> CCAGGCC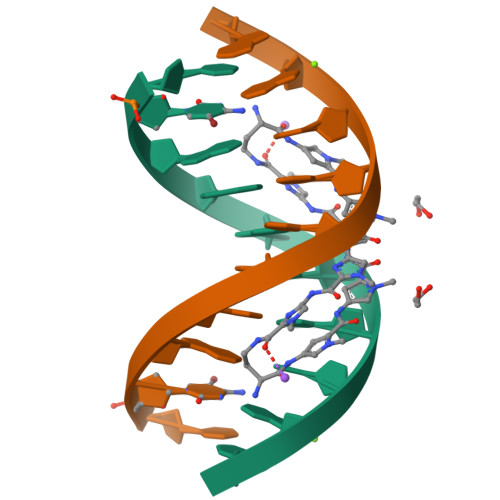TGG> 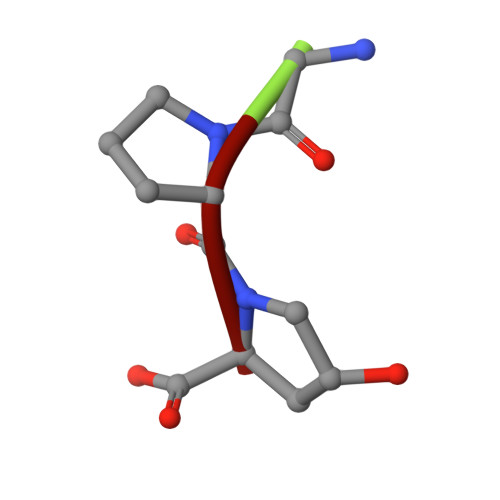GPP4-[(2R)-2-[(4-chlorobenzyl)oxy]-2-(2,4-dichlorophenyl)ethyl]-1H-imidazole 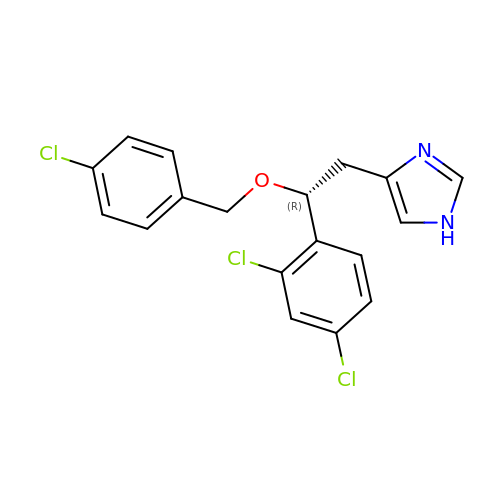| C18 H15 Cl3 N2 O | YYOREPIIQIKCGZ-GOSISDBHSA-N>[2x]RKIPKVGHTFFQKPESCPPVPGGSMKLDIGIINENQRVSMSRNIESRSTSPWNYTVTWDPNRYPSEVVQAQCRNLGCINAQGKEDISMNSVPIQQETLVVRRKHQGCSVSFQLEKVLVTVGCTCVTPVIHHVQ;> SLRLLDHRALVCSQPGLNCTVKNSTCLDDSWIHPRNLTPSSPKDLQIQLHFAHTQQGDLFPVAHIEWTLQTDASILYLEGAEL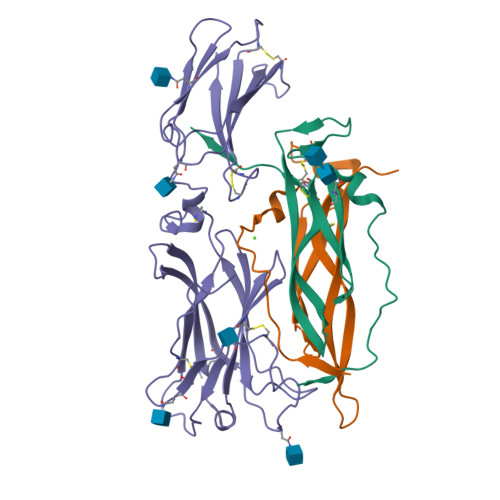SVLQLNTNERLCVRFEFLSKLRHHHRRWRFTFSHFVVDPDQEYEVTVHHLPKPIPDGDPNHQSKNFLVPDCEHARMKVTTPCMSSGSLWDPNITVETLEAHQLRVSFTLWNESTHYQILLTSFPHMENHSCFEHMHHIPAPRPEEFHQRSNVTLTLRNLKGCCRHQVQIQPFFSSCLNDCLRHSATVSCPEMPDTPEPIPDYM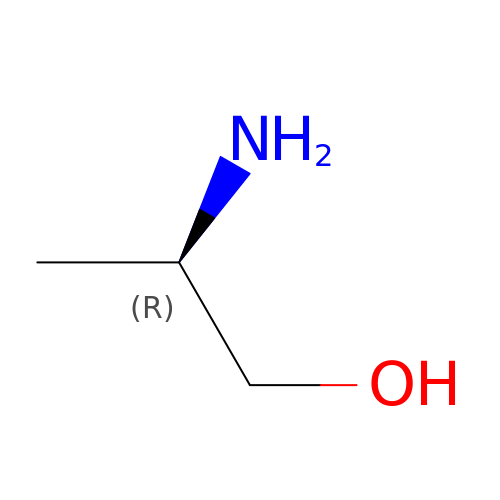(2R)-2-aminopropan-1-ol | C3 H9 N O | BKMMTJMQCTUHRP-GSVOUGTGSA-N>RKPRGRPKKX[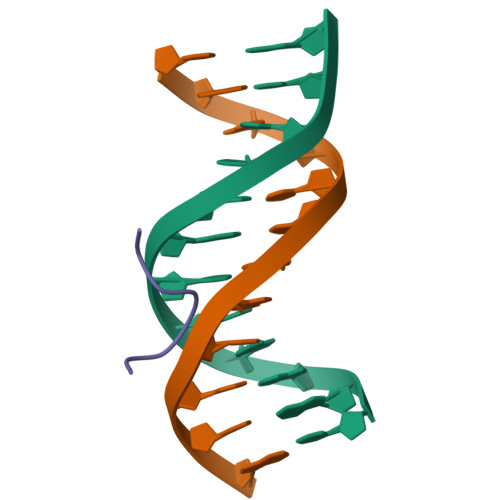4x]>MKKVALVTGAGQGIGKAIALRLV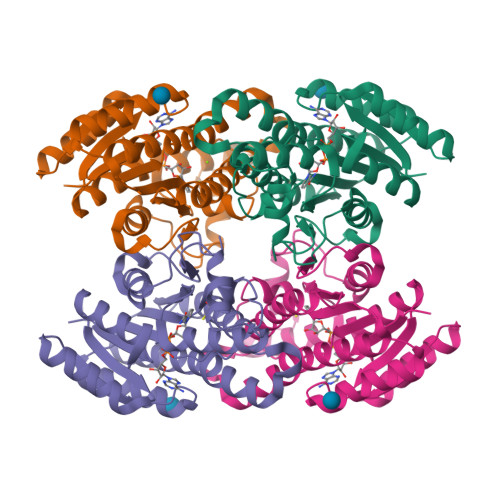KDGFAVAIADYNDATAKAVASEINQAGGHAVAVKVDVSDRDQVFAAVEQARKTLGGFDVIVNNAGVAPSTPIESITPEIVDKVYNINVKGVIWGIQAAVEAFKKEGHGGKIINACSQAGHVGNPELAVYSSSKFAVRGLTQTAARDLAPLGITVNGYCPGIVKTPMWAEIDRQVSEAAGKPLGYGTAEFAKRITLGRLSEPEDVAACVSYLASPDSDYMTGQSLLIDGGMVFN[8x]>[4x]MVNVAVIGAAGGIGQSLSLLLLRELPFGSTLSLYDVVGAPGVAADLSHIDRAGITVKHAAGKLPPVPRDPALTELAEGVDVFVIVAGVPRKPGMTRDDLFNVNAGIVMDLVLTCASVSPNACFCIVTNPVNSTTPIAAQTLRKIGVYNKNKLLGVSLLDGLRATRFINNARHPLVVPYVPVVGGHSDVTIVPLYSQIPGPLPDESTLKEIRKRVQVAGTEVVKAKAGRGSATLSMAEAGARFTMHVVKALMGLDTPMVYAYVDTDGEHECPFLAMPVVLGKNGIERRLPIGPITTVEKEMLEEAVGVVKKNIAKGETFARSKL;> MDCSTGAAIGQQFAKDAFHMHGGVGVGPTGNSEHDVLMNEMMMVQTPTGPAGEWTHQFAAYQGQQQQQQQQHPQELAMRHQQNDAFMLRQQQEMEEAFCTFCTTHPHSHAHSHQPQGLVGPAMMGPQIMPPMMFGPGTGGFMMGAPPMMPYASMK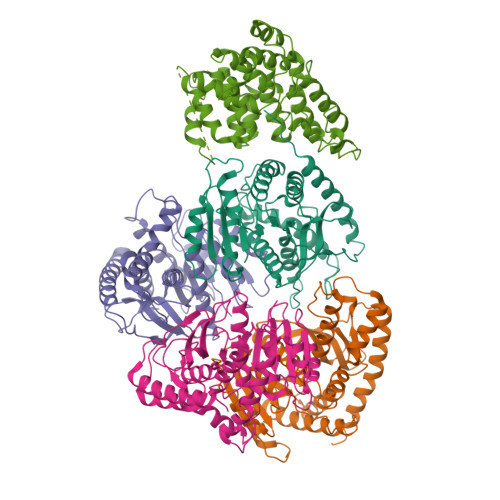FAGDAAMAAANNTNMTQGATATSTTSVQQELQQQSSDNGWVEKLRDAEWAQDYSDAQVFTLEGQSEQTMEEHAKNSEFYQFMDKIRSKELLIDEETGQLVQGPGPDPDAPEDAEYLKEWAAAEGLNMPPGFFEHMMQRPQGNNEQAEGRLFDGSNDALMDDGALDNAADVEEWVREYAEAQEQLQRVQNETNYPFEPNNPYMYHDKPMEEGIAMLQLANMAEAALAFEAVCQKEPENVEAWRRLGTTQAENEKDCLAIIALNHARMLDPKDIAVHAALAVSHTNEHNVGAALQSLRSWLLSQPQYEHLGLVDLREVAADEGLDEVPEENYFFAAPSEYRDCCTLLYAAVEMNPNDPQLHASLGVLHNLSHRFDEAAKNFRRAVELRPDDAHMWNKLGATLANGNRPQEALEAYNRALDINPGYVRVMYNMAVSYSNMAQYPLAAKHITRAIALQAGGTNPQGEGSRIATRGLWDLLRMTLNLMDRSDLVEASWQQDLTPFLREFGLEEMAV>[2x]AMAKDSKAPVVEIFDERDGCTSAGSTGKASDAGEKGLLVKVSMQKVGYNAIMAKSVAASYMN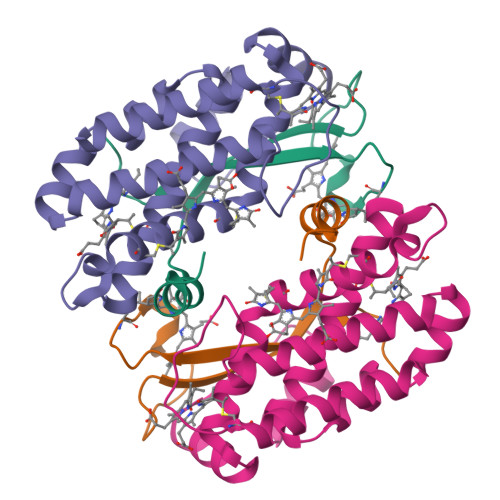A;>LDAFSKVITSADGKAAYVGGADLQALKKFVSDGNKRMDAVNAIVSNASCIVSDAVSGMVCENPSLIAPNGGVYSNRKMAACLRDAEIILRYVSYSLLSGDSSVLEDRCLNGLKETYSSLGVPAAGNARAVAIMKATVNSFINNTAQQKKLSVPSGDCSALASEAGGYFDKVTSAIA[2x]> MSEKTTKGVQLLRGDPKKAIVRLSIPMMIGMSVQTLYNLADGIWVSGLGPESLAAVGLFFPVFMGIIALAAGLGVGTSSAIARRIGARDKEGADNVAVHSLILSLILGVTITITMLPAIDSLFRSMGAKGEAVELAIEYARVLLAGAFIIVFNNVGNGILRGEGDANRAMLAMVLGSGLNIVLDPIFIYTLGFGVVGAAYATLLSMVVTSLFIAYWLFVKRDTYVDITLRDFSPSREILKDILRVGLPSSLSQLSMSIAMFFLNSVAITAGGENGVAVFTSAWRITMLGIVPILGMAAATTSVTGAAYGERNVEKLETAYLYAIKIAFMIELAVVAFIMLFAPQVAYLFTYSESAQVIKGDLISALRTLPVFLVLTPFGMMTSAMFQGIGEGEKSLILTIFRTLVMQVGFAYIFVHYTTLGLRGVWIGIV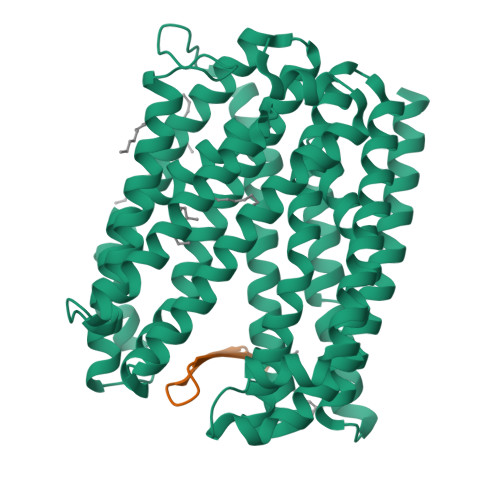IGNMVAAIVGFLWGRMRISALKKTSATGGKR;> AFTFRYSPSLYTWFLFPCG>[5x]EWTGDARDGMFSGVVITQFHTGQIDNKPYFCIEGKQSAGSSISACSMKNSSVWGASF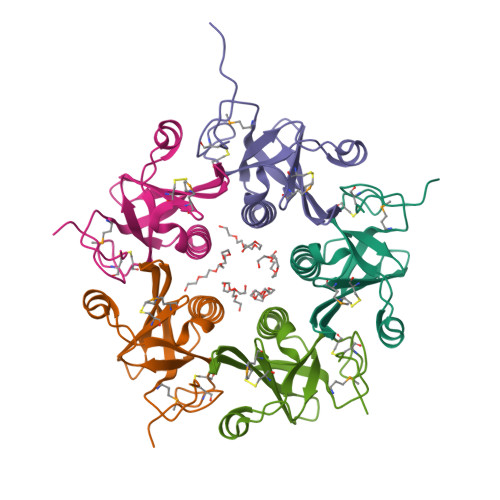STLYNQALYFYTTGQPVRIYYEPGVWTYPPFVKALTSNALVGLSTCTTSTECFGPDRKKNSLEHHHHHH> MDVFAKHAVSLESPAVRHYEITPSDSTDLARR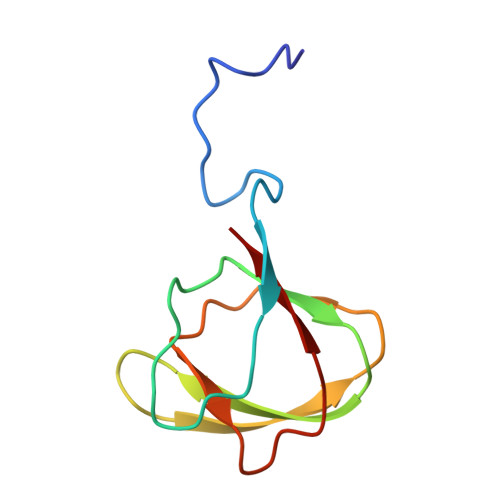PRALRVQTGGTLVLRDETGITVTYTVFAGEILPVRPVRVLATGTTATAVGWE> GGSDLDQGGEALAPRQVLDLEDLVFTQGSHFMANKRCQLPDGSFRRQRKGYEEVHVPALKPKPFGSEEQLLPVEKLPKYAQAGFEGFKTLNRIQSKLYRAALETDENLLLCAPTGAGKTNVALMCMLREIGKHINMDGTINVDDFKIIYIAPMRSLVQEMVGSFGKRLATYGITVAELTGDHQLCKEEISATQIIVCTPEKWDIITRKGGERTYTQLVRLIILDEIHLLHDDRGPVLEALVARAIRNIEMTQEDVRLIGLSATLPNYEDVATFLRVDPAKGLFYFDNSFRPVPLEQTYVGITEKKAIKRFQIMNEIVYEKIMEHAGKNQVLVFVHSRKETGKTARAIRDMCLEKDTLGLFLREGSASTEVLRTEAEQCKNLELKDLLPYGFAIHHAGMTRVDRTLVEDLFADKHIQVLVSTATLAWGVNLPAHTVIIKGTQVYSPEKGRWTELGALDILQMLGRAGRPQYDTKGEGILITSHGELQYYLSLLNQQLPIESQMVSKLPDMLNAEIVLGNVQNAKDAVNWLGYAYLYIRMLRSPTLYGISHDDLKGDPLLDQRRLDLVHTAALMLDKNNLVKYDKKTGNFQVTELGRIASHYYITNDTVQTYNQLLKPTLSEIELFRVFSLSSEFKNITVREEEKLELQKLLERVPIPVKESIEEPSAKINVLLQAFISQLKLEGFALMADMVYVTQSAGRLMRAIFEIVLNRGWAQLTDKTLNLCKMIDKR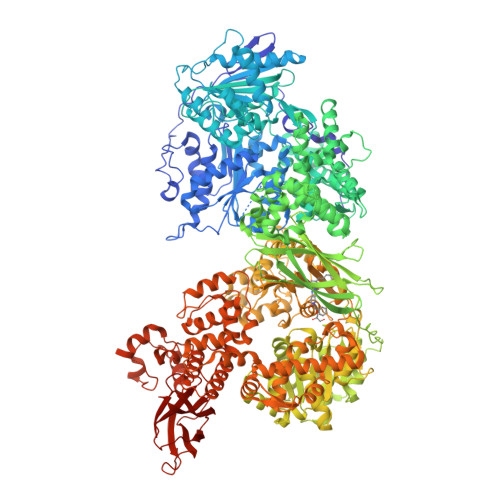MWQSMCPLRQFRKLPEEVVKKIEKKNFPFERLYDLNHNEIGELIRMPKMGKTIHKYVHLFPKLELSVHLQPITRSTLKVELTITPDFQWDEKVHGSSEAFWILVEDVDSEVILHHEYFLLKAKYAQDEHLITFFVPVFEPLPPQYFIRVVSDRWLSCETQLPVSFRHLILPEKYPPPTELLDLQPLPVSALRNSAFESLYQDKFPFFNPIQTQVFNTVYNSDDNVFVGAPTGSGKTICAEFAILRMLLQSSEGRCVYITPMEALAEQVYMDWYEKFQDRLNKKVVLLTGETSTDLKLLGKGNIIISTPEKWDILSRRWKQRKNVQNINLFVVDEVHLIGGENGPVLEVICSRMRYISSQIERPIRIVALSSSLSNAKDVAHWLGCSATSTFNFHPNVRPVPLELHIQGFNISHTQTRLLSMAKPVYHAITKHSPKKPVIVFVPSRKQTRLTAIDILTTCAADIQRQRFLHCTEKDLIPYLEKLSDSTLKETLLNGVGYLHEGLSPMERRLVEQLFSSGAIQVVVASRSLCWGMNVAAHLVIIMDTQYYNGKIHAYVDYPIYDVLQMVGHANRPLQDDEGRCVIMCQGSKKDFFKKFLYEPLPVESHLDHCMHDHFNAEIVTKTIENKQDAVDYLTWTFLYRRMTQNPNYYNLQGISHRHLSDHLSELVEQTLSDLEQSKCISIEDEMDVAPLNLGMIAAYYYINYTTIELFSMSLNAKTKVRGLIEIISNAAEYENIPIRHHEDNLLRQLAQKVPHKLNNPKFNDPHVKTNLLLQAHLSRMQLSAELQSDTEEILSKAIRLIQACVDVLSSNGWLSPALAAMELAQMVTQAMWSKDSYLKQLPHFTSEHIKRCTDKGVESVFDIMEMEDEERNALLQLTDSQIADVARFCNRYPNIELSYEVVDKDSIRSGGPVVVLVQLEREEEVTGPVIAPLFPQKREEGWWVVIGDAKSNSLISIKRLTLQQKAKVKLDFVAPATGAHNYTLYFMSDAYMGCDQEYKFSVDVKEA>[4x]MGSSHHHHHHSSGLVPRGSHMTDLSDVSRTAAAKPPAVPGRGPANKVRFVTAASLFDGHDASINIMRRILQSQGCEVIHLGHNRSVQEVVTAALQEDVQGIAISSYQGGHVEYFKYMIDLLREHGGEHIQVFGGGGGVIVPDEIRELQAYGVARIYSPEDGQRMGLAGMITDMAQRCDIDLTRYAPTTLDTVVAGDRRALAQLITALENGKADPELVSALHAQAKAAAVPVLGITGTGGAGKSSLTDELIRRFRLDQDDALSIAVISIDPSRRKSGGALLGDRIRMNAINHPNIFMRSLATREAGSEISQALPDVIAACKAARFDLVIVETSGIGQGDAAIVPHVDLSLYVMTPEFGAASQLEKIDMLDFADFVAINKFDRKGAQDAWRDVAKQVQRNREQWHSRAEDMPVYGTQASRFNDDGVTMLYQGLVGALGARGMSLKPGTLPNLEGRISTGQNVIVPPARSRYLAELADTVRAYHRRVVAQSKLARERQQLRAAHDMLQGAGHESAALETLASERDVSLGAVERKLLAMWPQMQQAYSGDEYVVKIRDKEIRTGLISTTLSGTKIRKVVLPRFEDEGEILKWLMRENVPGSFPYTAGVFAFKREGEDPTRMFAGEGDAFRTNRRFKLVSEGMEAKRLSTAFDSVTLYGEDPHERPDIYGKVGNSGVSIATLEDMKVLYDGFDLTNPSTSVSMTINGPAPTILAMFMNTAIDQQIDRFRADNGRDPTADEEAKIRAWVLQNVRGTVQADILKEDQGQNTCIFSTEFSLKVMGDIQEYFVHHQVRNFYSVSISGYHIAEAGANPISQLAFTLANGFTYVEAYLARGMHIDDFAPNLSFFFSNGMDPEYSVLGRVARRIWAVTMRDKYGANDRSQKLKYHIQTSGRSLHAQEIDFNDIRTTLQALIAIYDNCNSLHTNAYDEAITTPTAESVRRALAIQLIINREWGVAKCENPNQGSFLIEELTDLVEEAVLQEFERIAERGGVLGAMETGYQRGKIQEESLYYEQLKHDGTLPIIGVNTFRNPNGDPTPQTLELARSSEDEKQSQLHRLTEFHGAHQADAEAMLARLRQAVIDNRNVFAVLMDAVRVCSLGQITHALFEVGGQYRRNM

Although most chaperones are standalone proteins, isobutyryl-CoA mutase fused (IcmF) has a G-protein domain covalently attached to its target mutase. IcmF catalyzes the 1,2-rearrangement of isobutyryl-CoA to n-butyryl-CoA, as well as pivalyl-CoA and isovaleryl-CoA, using AdoCbl. Here, we show that the G-protein domain in a fused system forms a similar active conformation, requiring IcmF oligomerization. Cryo-EM structural analysis reveals that the second protomer of the G-protein intermolecular dimer props open the mutase active site using residues of switch III as a wedge, allowing for AdoCbl insertion or damaged Cbl removal.

With 500 μM of the nonhydrolyzable GTP analog, GMPPCP, long chains of IcmF protomers are observed, with all visible IcmF protomers comprising these filamentous-like chains. To further investigate the structures of IcmF’s supramolecular complexes, we prepared cryogenic EM grids and collected datasets of C. metallidurans wt IcmF with GMPPCP and butyryl-CoA (wt IcmF + GMPPCP) and Q341A IcmF with GTP (Q341A IcmF + GTP). For the wt IcmF + GMPPCP dataset, the supramolecular complexes were first manually picked on the micrographs, extracted using helical parameters, and processed as a single particle dataset. Signal subtraction was utilized to remove the extra density that was due to the extraction of single particles from a continuous helical particle. Local B factor postprocessing was performed to yield a 6.7-Å resolution reconstruction. However, due to the lower resolution of the wt IcmF + GMPPCP reconstruction, there is no clear density for GMPPCP in the nucleotide-binding site. The G-protein domain interface adopts the same conformation as observed for MeaB in the GMPPCP-MeaB:MCMCbl complex structure. For both reconstructions, we observed an open conformation of the mutase active site. In terms of maturation, the formation of the supramolecular complexes made up of apo-IcmF molecules with GMPPCP (right) invokes an assembly line model in which a chain of open mutases can be filled in succession by an ATR that moves down the chain, delivering AdoCbl as it is synthesized.The three-finger toxin (3FT) family is widely represented as structural motif, mainly in the Elapidae snake venoms, supporting various biological functions. This fold is characterized by three adjacent loops rich in β-pleated sheets emerging from a small globular core containing four invariant disulfide bridges. Despite high primary structure identity, often greater than 55%, muscarinic and adrenergic toxins exhibit distinct pharmacological profiles and clear functional differences. “Loop grafting” has been used to construct seven chimeric toxins to dissect how the affinity, selectivity and functionality for the muscarinic and adrenergic receptors depend on shuffling loops between various toxins.

On the other hand, the mode of interaction of MT1 with muscarinic receptors is less precisely defined, but its selectivity profile for M1 and M4 receptors has been clearly established (review in [20], [21]). Based on previous data reporting adrenergic effects of MT1 in tissue preparations, the ability of various MTs to interact with adrenoceptors was investigated, showing that MT1 interacts efficiently with mAChRs and also with α1A- and α2B-adrenoceptors. The comparisons of loop 2 from MT1 and MT7 shows that the backbone of this loop is conserved between the two natural toxins, but the side chains adopt a different orientation. Another invariable is that the backbone conformation of loop 2 is well conserved between MT7 and MT1, although the sequence is not. MT1 superimposition onto MT7 by least-squares fit shows large deviations in both the loops and in the sequence-conserved disulphide-bridged scaffold leading to important differences when the main chain atoms are compared (rmsd MT1 vs MT7 = 3.22±0.01 Å, depending on the molecule in the asymmetric unit that are compared). A better match can be obtained by not matching consecutive residues but only the secondary-structure elements. Secondary-structure matching (SSM) for the MT1/MT7 comparison leads to a value of around 1.34 Å where the matched residues have a reduced sequence identity of only 66%. The affinity of MT7 for hM4 is very low (pKi: 4.87±0.06), approximately 40-fold less than that of MT1 (pKi: 6.50±0.04). Equilibrium binding experiments with [3H]-Prazosin show that MT1 and MT7 toxins interact with α1A-adrenoceptor with relatively high (pKi: 7.21±0.16) and very low affinity (pKi >4.7), respectively. The tip of this loop is relatively independent of the rest of the toxin in MT7 but in MT1 with the longer loop 3 this is no longer the case.

>[2x]LTCVTSKSIFGITTENCPDGQNLCFKKWYYIVPRYSDITWGCAATCPKPTNVRETIRCCETDKCNE tetrazolo[5,1-b]quinazolin-9-ol | C8 H5 N5 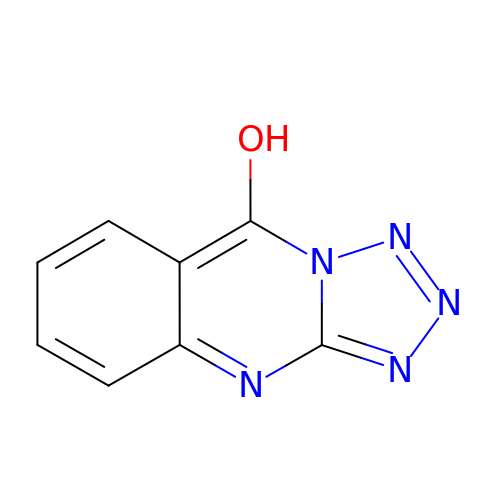O | MBODJNHSMUWROS-UHFFFAOYSA-N>GSHMNGNNTSETQGDRTEQAETVQADLFSADSAYTFVQRQVNFGPRIPGTAPHRACGDWLVATLRSFGAAVQEQTAEIKAHDGTMLPMRNIIASYRPEATGRMLLMAHWDTRPVCDQDANPAMHTETFDGADDGGSGVGVLLEIARYLGQQKDLGMGIDIVFFDTEDYGSYGDDESWCLGSQYWSRNPHVAGYKAEAGILLDMVGAKGATFYWEYFSKSYAPGLISAVWQTAAALGYGNYFIQADGGALTDDHVPVIKNLGIPCIDIINYSSKNEHGFGDHWHTQRDNMQIIDKNVLDAVGETVIRYLDEQVKAASH[2x]

QCs belong to the family of aminoacyltransferases and catalyze the cyclization of N-terminal glutamine/glutamate residues of peptides and proteins with concomitant release of ammonia/water. Glutaminyl cyclases (QCs) from the oral pathogens Porphyromonas gingivalis, Tannerella forsythia, and Prevotella intermedia represent attractive target enzymes for small-molecule inhibitor development, as their action is likely to stabilize essential periplasmic and outer membrane proteins by N-terminal pyroglutamination. Crystal structures of the enzymes from P. gingivalis (PgQC) and T. forsythia (TfQC) reveal a tertiary structure composed of an eight-stranded β-sheet surrounded by seven α-helices, typical of animal type II QCs. In each case, an active site Zn ion is tetrahedrally coordinated by conserved residues.

PgQC crystallized in a trigonal crystal form with two monomers in the asymmetric unit. Both monomers display a compact architecture of the type II QC α/β-hydrolase fold: an open-sandwich topology with a twisted central six-stranded β-sheet βA–βB–βC–βD–βE–βH (with βB running antiparallel to the others), surrounded on the concave side by helices α6 and α8, on the convex side by α2, α3, α4, and α9, and closed on one edge by the segment βF–α7’–α7–βG. Several of the loops connecting secondary structure elements are shorter compared with HsQC, as are helices α6 and α7, and helix α5 is missing altogether. In contrast, helix α7 of PgQC, which is shifted by half a pitch compared with its HsQC counterpart, is preceded by the short helix α7’. The single-zinc active site of PgQC bears a strong resemblance to that of animal QCs. Replacement of the third zinc ligand (HsGlu202) with the shorter PgAsp183 results in a minor rearrangement of the main chain. Of note, the indole ring of PgTrp193 (conserved in bacteroidal QCs,), which is C terminal to the “insertion loop” and prior to α6, occupies a similar spatial position to that of HsTrp207, which forms one edge of the active site pocket and has been shown to participate in substrate binding and catalysis. As a result of a different main chain position of PgTrp193 and resulting side chain orientation, the active site is much deeper than in animal QCs. Access is further restricted by (i) the loop following strand βC formed by residues PgArg128, PgPro129, and PgAsp132 (all conserved in bacteroidal QCs), (ii) the inserted loop following βH immediately prior to PgPhe294 and PgTrp298 (both conserved in all type II QCs and that presumably play a role in substrate binding), as well as (iii) the extended chain between βG and α8 that shows structural variability in TfQC and in mammalian QCs.>[3x]MLHHHHHHPMGRGTITDASGFDPLRDAEVLRKAMKGFGTDEQAIIDCLGSRSNKQRQQILLSFKTAYGKDLIKDLKSELSGNFEKTILALMKTPVLFDVYEIKEAIKGAGTDEACLIEILASRSNEHIRELNRAYKTEFKKTLEEAIRSDTSGHFQRLLISLSQGNRDESTNVDMSLVQRDVQELYAAGENRLGTDESKFNAILCSRSRAHLVAVFNEYQRMTGRDIEKSICREMSGDLEQGMLAVVKCLKNTPAFFAERLNKAMRGAGTKDRTLIRIMVSRSELDLLDIRAEYKRMYGKSLYHDITGDTSGDYRKILLKICGGND

The annexin (Anx) family of Ca2+-binding proteins is widely distributed in eukaryotes, with twelve Anxs found in vertebrates. The Anxs are structurally distinct from the EF-hand and C2-domain Ca2+-binding proteins. They reversibly bind negatively charged lipids in a Ca2+-dependent manner, which is a defining feature of this protein family. AnxA11 has the longest N-terminal domain of all Anxs, with ~200 residues. Recent studies have revealed that mutations in AnxA11 play an important role in the development of the neurodegenerative disease amyotrophic lateral sclerosis (ALS).

Since the long N terminus of AnxA11 renders recombinant production of the protein challenging, N-terminally truncated recombinant forms were generated, and the crystal structure of one form, Δ188AnxA11, was determined. Using Δ188AnxA11, we solved the crystal structure of the rat AnxA11 core domain. The asymmetric unit contains three molecules of AnxA11, and the structure presents the canonical Anx core fold. The Ca2+ binding sites are partially occupied, whereby two monomers have three Ca2+ ions bound, and one monomer has four. As is typical for the Anxs, all Ca2+ binding sites are on one face of the molecule, promoting calcium-dependent lipid membrane binding. We show that a 4-residue sequence motif in the N terminus of the core structure, conserved in most Anxs, functions as a Velcro-like bridging segment and is important for the thermal stability of the Anx core structure. The substantial difference in thermal stability induced by the four N-terminal residues of the Δ188AnxA11 construct implies an important structural element at this position. This segment, ~10 residues before the AnxA11 domain I helix A, is central in the folded structure, making interactions with the termini of several helices of the Anx fold, and effectively enabling a tight contact between the N terminus of domain I and the C terminus of domain IV. The 4-residue segment forms conserved interactions with the ends of helices in domain IV. The crystal structure of AnxA11 presents trimers very similar to those formed by AnxA5, and hence, could be expected to interact with membranes in a similar manner. Interestingly, three of these mutations involve a buried Arg residue, and a close look at the alignment reveals that these Arg residues are fully conserved in all rat Anxs.> MVPISPIETVPVKLKPGMDGPKVKQWPLTEEKIKALVEICTEMEKEGKISKIGPENPYNTPVFAIKKKDSTKWRKLVDFRELNKRTQDFWEVQLGIPHPAGLKKKKSVTVLDVGDAYFSVPLDEDFRKYTAFTIPSINNETPGIRYQYNVLPQGWKGSPAIFQSSMTKILEPFAAQNPDIVIYQYMDDLYVGSDLEIGQHRTKIEELRQHLLRWGLTTPDKKHQKEPPFLWMGYELHPDKWTVQPIVLPEKDSWTVNDIQKLVGKLNWASQIYPGIKVRQLSKLLRGTKALTEVIPLTEEAELELAENREILKEPVHGVYYDPSKDLIAEIQKQGQGQWTYQIYQEPFKNLKTGKYARMRGAHTNDVKQLTEAVQKITTESIVIWGKTPKFKLPIQKETWETWWTEYWQATWIPEWEFVNTPPLVKLWYQLEKEPIVGAETFYVDGAANRE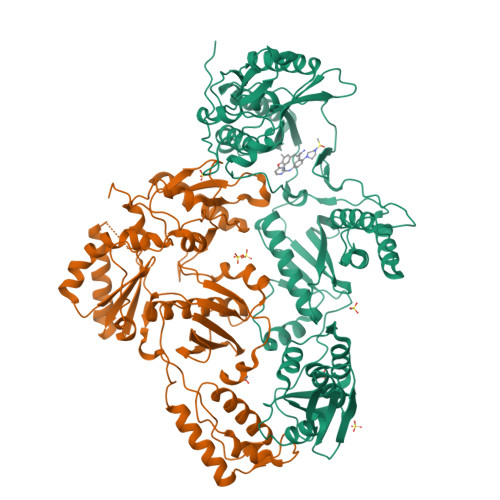TKLGKAGYVTNKGRQKVVPLTNTTNQKTELQAIYLALQDSGLEVNIVTDSQYALGIIQAQPDKSESELVNQIIEQLIKKEKVYLAWVPAHKGIGGNEQVDKLVSAG;> GPISPIETVPVKLKPGMDGPKVKQWPLTEEKIKALVEICTEMEKEGKISKIGPENPYNTPVFAIKKKDSTKWRKLVDFRELNKRTQDFWEVQLGIPHPAGLKKKKSVTVLDVGDAYFSVPLDEDFRKYTAFTIPSINNETPGIRYQYNVLPQGWKGSPAIFQSSMTKILEPFKKQNPDIVIYQYMDDLYVGSDLEIGQHRTKIEELRQHLLRWGLTTPDKKHQKEPPFLWMGYELHPDKWTVQPIVLPEKDSWTVNDIQKLVGKLNWASQIYPGIKVRQLSKLLRGTKALTEVIPLTEEAELELAENREILKEPVHGVYYDPSKDLIAEIQKQGQGQWTYQIYQEPFKNLKTGKYARMRGAHTNDVKQLTEAVQKITTESIVIWGKTPKFKLPIQKETWETWWTEYWQATWIPEWEFVNTPPLVKLWYQ> SMNTDPLLPGFDYLTLHTSAARLRVAVKGSGPPLLLLHGYPQTHLAWHRIAPRLAEDYSVVLADL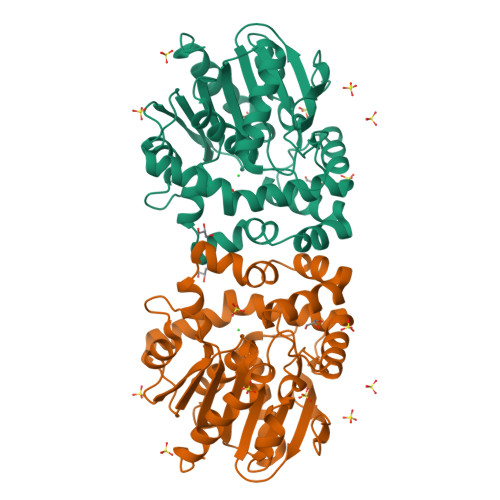RGYGESRALDEEGADYSKAALARDQLETMGQLGFERFAVIGHDRGARVGYRLALDHPQAVAAFVSLDVVPILDNWAAVNKVFALNAYHWFLLAQPYDLPERLIGADPEHFLDYTLRRMAQGRDIYHPQALESYRRAFRDPAVRHAMCEDYRAAVGVDADADQADRDAGRRLQCPVQVLWQERPYAAGQHPLEIWKTWAGQVEGAAIGASHMLPEDAPDAVLEHLLGFLASHREALR> MWDVIDLSRWQFALTALYHFLFVPLTLGLIFLLAIMETIYVVTGKTIYRDMTRFWGKLFGINFALGVATGLTMEFQFGTNWSFYSNYVGDIFGAPLAMEALMAFFLESTFVGLFFFGWQRLNKYQHLLVTWLVAFGSNLSALWILNANGWMQYPTGAHFDIDTLRMEMTSFSELVFNPVSQVKFVHTVMAGYVTGAMFIMAISAWYLLRGRERNVALRSFAIGSVFGTLAIIGTLQLGDSSAYEVAQVQPVKLAAMEGEWQTEPAPAPFHVVAWPEQDQERNAFALKIPALLGILATHSLDKPVPGLKNLMAETYPRLQRGRMAWLLMQEISQGNREPHVLQAFRGLEGDLGYGMLLSRYAPDMNHVTAAQYQAAMRGAIPQVAPVFWSFRIMVGCGSLLLLVMLIALVQTLRGKIDQHRWVLKMALWSL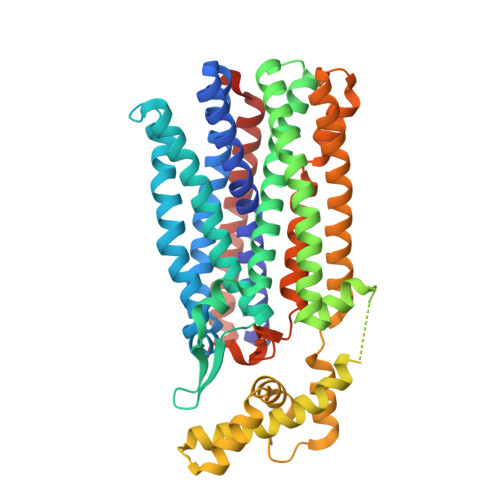PLPWIAIEAGWFMTEFGRQPWAIQDILPTYSAHSALTTGQLAFSLIMIVGLYTLFLIAEVYLMQKYARLGPSAMQSEQPTQQQG>[6x]MVYVNSVCHMKAAATAGKVEGEGDMQKKFPLAAISKVITTLWAIEKLGVDYRHKTVLHLTPTANGSMDLHVEGSRDPIFGRNLSYFLISELNRMKVTKIENLTFDENFLLDWLAEESPRIGGVTPRYETIEQQAEAVIKNLKESFSTAINRAMYSKLRERATKAKVFMLEKPTIEVRNISFLPKNNYKKDKYTGSVVLQSAPLRTILKRMNNQSNNYIADNLYWNLGGTAAFNAFAAATLKADQNQIVFHNGSGNNEGTTAK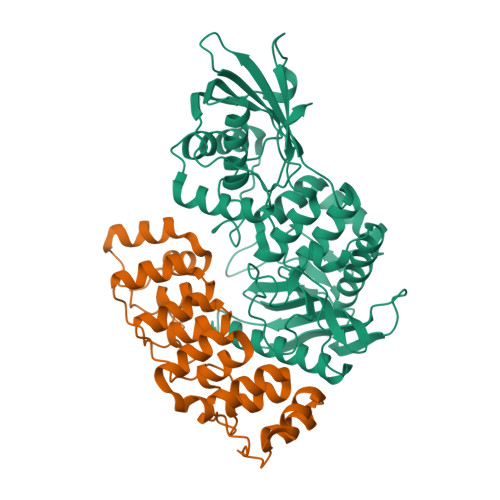PIYNEATCETMIKTLYTLNKSLEAKGYKLSDVLSVANKDSDSTIDNFGGNAAGSMIAKTGTVNKAKTLAGSISTKEGEFYFAILLHTDMDQSSSDRGVASQMIKNKISQLINKRSGPKEIQYTEILALPFDQNSYLTEA;>KSSKALNEAAEQGDLAKVKNLVQKNKIDLNAQDETGMTPLMNAAMGGNLDIVKFLLSKKVNLELKNNGGETALAFAVTNDAYDVAEELIKAGANVDIIVAGDEGDTLFMRAAQNNKKTAESILAKNKSLINKANTLGETALFAVARYGTPADIDFLIKKGADLKLKNKKGQTALDVAKEASNQDTAKALSKKK[6x]>GPGSMSAENTSTDADPTAHWSFETKQIHAGQQPDSATNARALPIYQTTSYTFENTAHAAALFGLEVPGNIYTRLGNPTTDVVEQRIAALEGGVAALFLSSGQAAETFAILNLAGAGDHIVSSPRLYGGTYNLFHYSLAKLGIEVSFVDDPDNLDSWQAAVRPNTKAFFGETISNPQIDLLDTPGVAEVAHRNGIPLIVDNTIATPYLIRPFTQGADIVVHSATKYLGGHGAAIAGVIVDGGTFDWTQGRFPEFTTPDPSYHGVVFAELGAPAYALKARVQLLRDLGSAASPFNAFLVA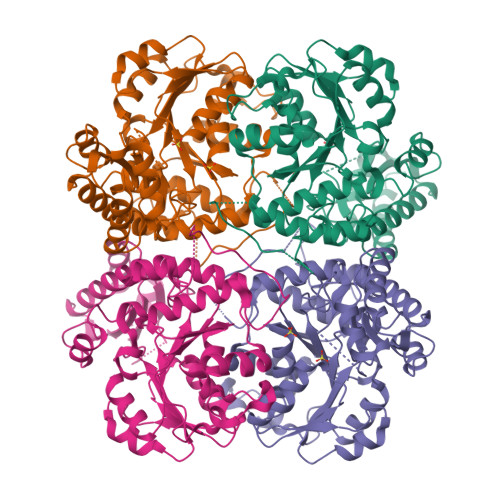QGLETLSLRIERHVSNAQRVAEFLADREDVVTVNYAGLPGSPWHERAKKLSPKGTGAVLSFELAGGVEAGKAFVNALKLHSHVANIGDVRSLVIHPASTTHAQLSPAEQLSTGVSPGLVRLAVGIEGIEDILADLELGFAAARKFSGDSQAVAAI[4x]1-methylethyl 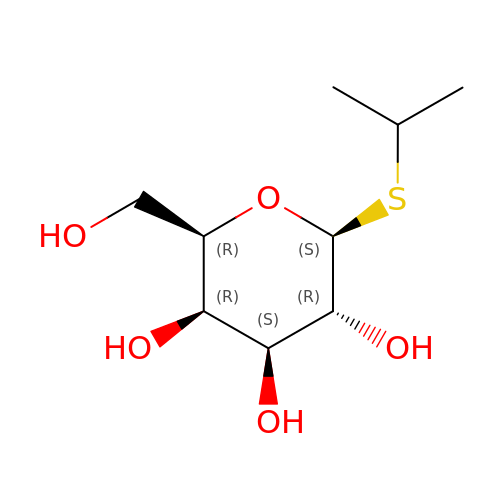1-thio-beta-D-galactopyranoside | C9 H18 O5 S | BPHPUYQFMNQIOC-NXRLNHOXSA-N>[2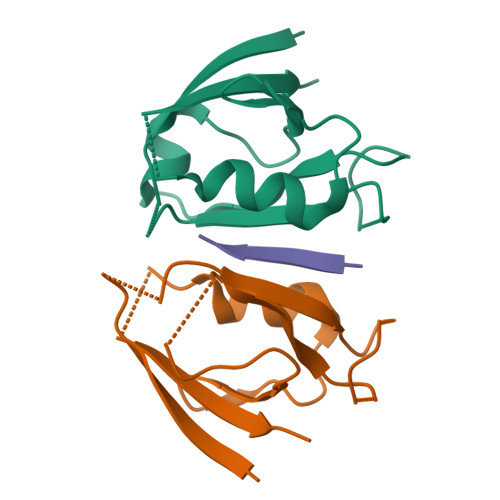x]SVEEIRLPRAGGPLGLSIVGGSDHSSHPFGVQEPGVFISKVLPRGLAARSGLRVGDRILAVNGQDVRDATHQEAVSALLRPCLELSLLVRRD;> LRLESSII>MKFSVIVPTYNSEKYITELLNSLAKQDFPKTEFEVVVVDDCSTDQTLQIVEKYRNKLNLKVSQLETNSGGPGKPRNVALKQAEGEFVLFVDSDDYINKETLKDAAAFIDEHHSDVLLIKMKGVNGRGVPQSMFKETAPEVTLLNSRIIYTLSPTKIYRTALLKDND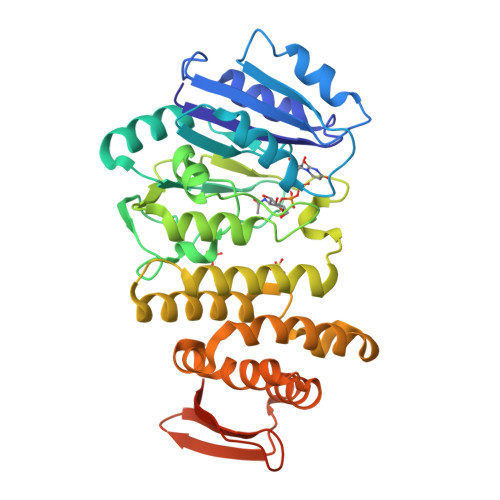IYFPEELKSAEDQLFTMKAYLNANRISVLSDKAYYYATKREGEHMSSAYVSPEDFYEVMRLIAVEILNADLEEAHKDQILAEFLNRHFSFSRTNGFSLKVKLEEQPQWINALGDFIQAVPERVDALVMSKLRPLLHYARAKDIDNYRTVEESYRQGQYYRFDIVDGKLNIQFNEGEPYFEGIDKLVPRGSAAAALEHHHHHH[2x]6-{2-amino-6-[(3R)-3-methylmorpholin-4-yl]pyrimidin-4-yl}-2H-indazol-3-amine 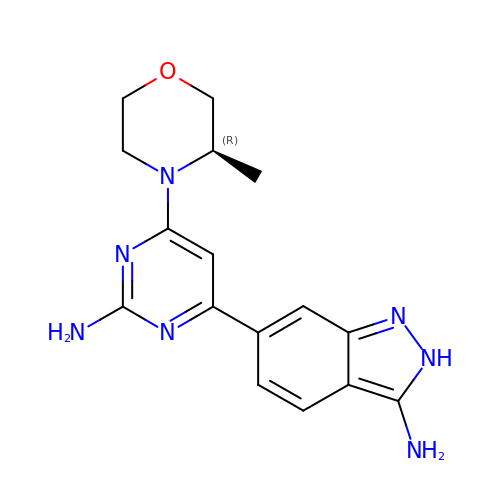| C16 H19 N7 O | WNVXQKKSIHKYCX-SECBINFHSA-N> MPQYQTWEEFSRAAEKLYLADPMKARVVLKYRHSDGNLCVKVTDDLVCLVYKTDQAQDVKKIEKFHSQLMRLMVAKEARNVTM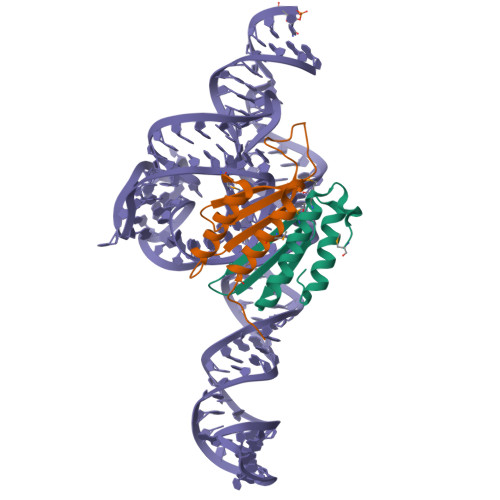ET;> MVLLESEQFLTELTRLFQKCRTSGSVYITLKKYDGRTKPIPKKGTVEGFEPADNKCLLRATDGKKKISTVVSSKEVNKFQMAYSNLLRANMDGLKKRDKKNKTKKTK>[2x]SLMAGLPNSSNALQQWHHLFEAEGTKRSPQAQQHLQQLLRTGLPTRKHENWKYTPLEGLINSQFVSIAGEI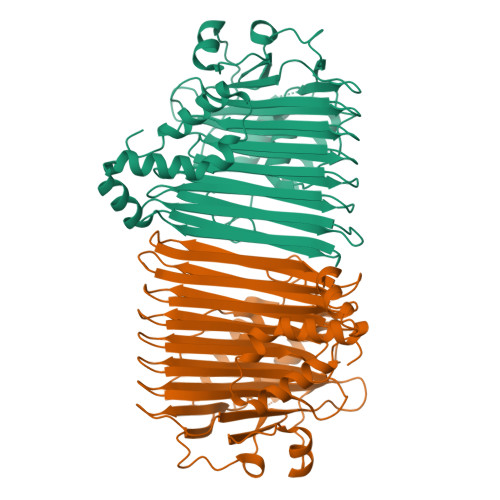SPQQRDALALTLDSVRLVFVDGRYVPALSDATEGSGYEVSINDDRQGLPDAIQAEVFLHLTESLAQSVTHIAVKRGQRPAKPLLLMHITQGVAGEEVNTAHYRHHLDLAEGAEATVIEHFVSLNDARHFTGARFTINVAANAHLQHIKLAFENPLSHHFAHNDLLLAEDATAFSHSFLLGGAVLRHNTSTQLNGENSTLRINSLAMPVKNEVCDTRTWLEHNKGFCNSRQLHKTIVSDKGRAVFNGLINVAQHAIKTDGQMTNNNLLMGKLAEVDTKPQLEIYADDVKCSHGATVGRIDDEQIFYLRSRGINQQDAQQMIIYAFAAELTEALRDEGLKQQVLARIGQRLPGGAREGGSHHHHHH8-chloro-2-[(2S)-pyrrolidin-2-yl][1]benzofuro[3,2-d]pyrimidin-4(3H)-one | C14 H12 Cl N3 O2 | 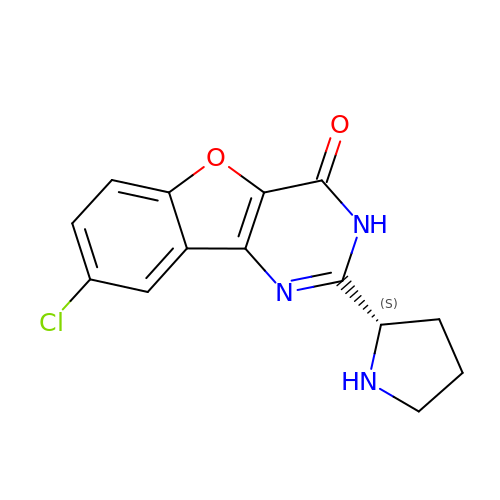JJWLXRKVUJDJKG-VIFPVBQESA-N>GDPNQAVLKFTTEIHPSCVTRQKVIGAGEFGEVYKGMLKTSSGKKEVPVAIKTLKAGYTEKQRVDFLGEAGIMGQFSHHNIIRLEGVISKYKPMMIITEYMENGALDKFLREKDGEFSVLQLVGMLRGIAAGMKYLANMNYVHRDLAARNILVNSNLVCKVSDFGLSRVLEDDPEATYTTSGGKIPIRWTAPEAISYRKFTSASDVWSFGIVMWEVMTYGERPYWELSNHEVMKAINDGFRLPTPMDCPSAIYQLMMQCWQQERARRPKFADIVSILDKLIRA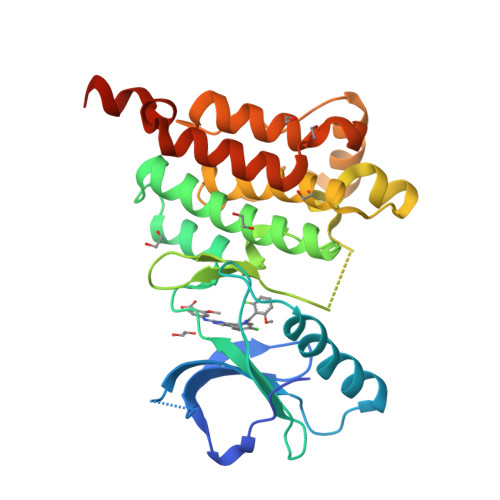PDSLKTLADFDPRVSIRLPSTSG[3x]>MSTPQDNANTVHRYLEFVAKGQPDEIAALYADDATVENPVGSEVHIGRQAIRGFYGNLENVQSRTEVKTLRALGHEVAFYWTLSIGGDEGGMTMD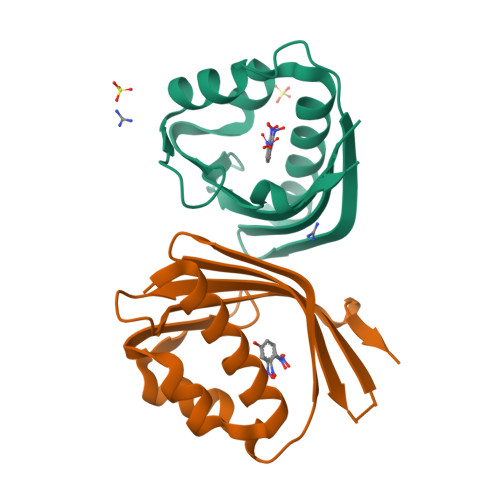IISVMTFNDDGRIKSMKAYWTPENITQR[2x]>MLTQHVSEARTRGAIHTARLIHTSDLDQETRDGARRMVIEAFRDPSGDSDFTDDFTDDDWDHALGGMHALISHHGALIAHGAVVQRRLMYRGPDGRGHALRCGYVEAVAVREDRRGDGLGTAVLDALEQVIRGAYQIGALSASDIARPMYIARGWL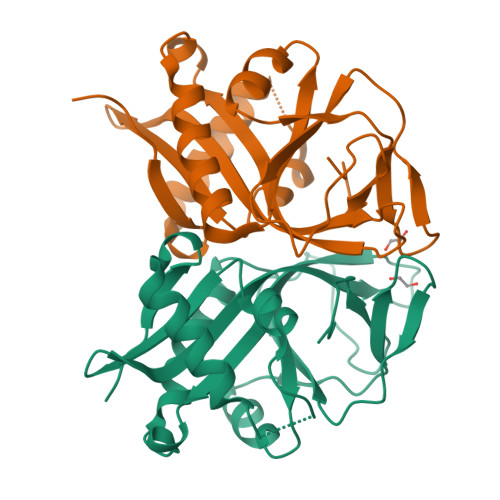SWEGPTSVLTPTEGIVRTPEDDRSLFVLPVDLPDGLELDTAREITCDWRSGDPW[4x]> MAELACFCYPHLENDSYKFI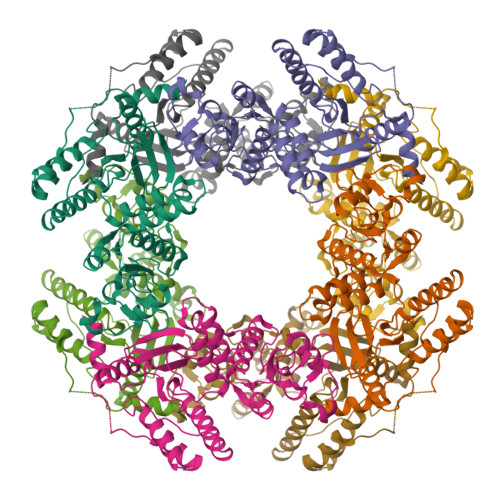PFNNLAIKAMLTAKVDKKDMDKFYDSIIYGIAPPPQFKKRYNTNDNSRGMNFETIMFTKVAMLICEALNSLKVTQANVSNVLSRVVSIRHLENLVIRKENPQDILFHSKDLLLKSTLIAIGQSKEIETTITAEGGEIVFQNAAFTMWKLTYLEHQLMPILDQNFIEYKVTLNEDKPISDVHVKELVAELRWQYNKFAVITHGKGHYRIVKYSSVANHADRVYATFKSNVKTGVNNDFNLLDQRIIWQNWYAFTSSMKQGNTLDVCKRLLFQKMEPEKNPFKGLSTDRKMDEVS>MSLLSDLCNLNLSESTEKIIAEYIWIGGSGMDLRSKARTLNAPVSDPSKLPQWNYDGSSTGQAPGEDSEVILYPQAIYKDPFRRGNNILVMCDAYTPGGEPIPTNKRFDAAKIFSHPDVVAEEPWYGIEQEYTLLQKEVKWPIGWPVGGYPGPQGPYYCGIGADKAFGRDIVDAHYKACLYAGINISGINGEVMPGQWEFQVGPSVGISSGDQLWMARYILERITEIAGVVVSFDPKPIEGDWNGAGAHTNYSTKSMRSDGGFEVI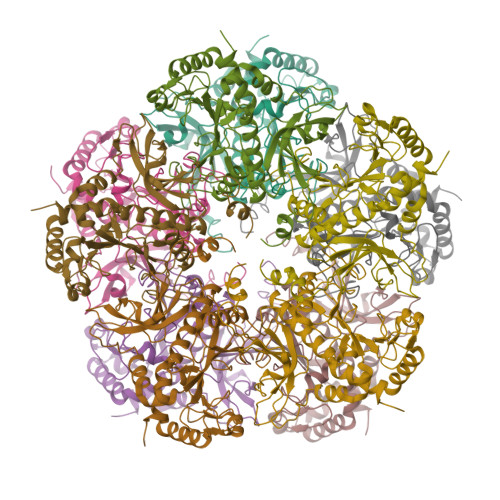KKAIEKLGLKHREHIAAYGEGNERRLTGKHETADINTFLWGVANRGASIRVGRDTEKAGKGYFEDRRPASNMDPYIVTSMIANTTILWKP[10x]>MGSDKIHHHHHHENLYFQGMFRPQDDFTYLMPVHFGGGKFDPETLVTQKATALSLSFETERDLLENYIPEGFELLAPEVQVAFNKFTEINWLHGGQYNLINVAAPVRFHGKKDELDGAYTLVVWENKTAPILGGREQTGIPKIYADIEDLHIVRPHFATTVSYEGNTFLNMDFEATGSITGRDLDALKSQFLTMNTLGWRYIPKVGAPGAELSQFVLYPQGMEVETAEVGKGSLKWTELTPMQSPAQYYIVNSLASLPIKRVTQAVLVEGRAI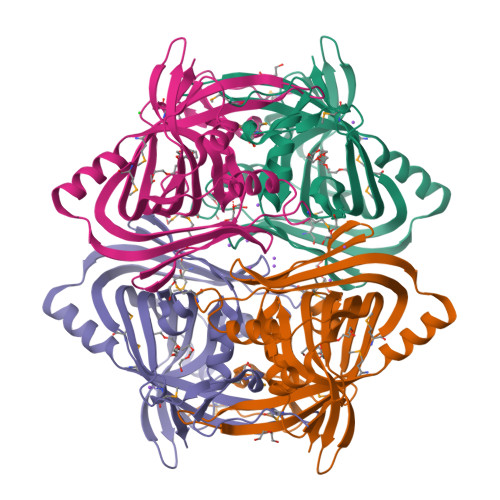LRAMGARVIE[4x]>MHHHHHHMIVRRATYEDLSQLAVLFDEYRQFYGASSNLEESHHFLKQRFENKESVFFIHIKDEKITGFVLLYLGFSSVACSTYYILDDVYVTPLFRRQGSAKQLIDTAILFAKQENALRISLETQSNNHESHRLYEKMGFIRDSEFQTFHCFLK[2x]

Here we have uncovered a GNAT-family acetyltransferase conserved in A. baumannii that is responsible for the acetylation of 1,3-DAP in A. baumannii in vivo and in vitro and renamed accordingly as Dpa for diamino-propane acetyltransferase. The crystal structure of Dpa reveals topological and functional differences from other bacterial polyamine acetyltransferases, adopting a β-swapped quaternary arrangement similar to that of eukaryotic polyamine acetyltransferases with a central size exclusion channel that sieves through the cellular polyamine pool. In this study, we have found a downstream regulatory element in this pathway: the polyamine acetyltransferase Dpa that specifically acetylates 1,3-DAP in A. baumannii to control the effective levels of the metabolite. The structure of Dpa revealed a dimeric architecture with a conserved acCoA and an acidic polyamine binding site formed at the dimer interface that shares properties with other polyamine acetyltransferases.

To better understand its structure-function interplay, we determined the structure of Dpa bound to acCoA. Dpa had an overall topology common to GNAT family acetyltransferases. Unlike SpeG acetyltransferases that form higher oligomers, Dpa formed a dimer through a C-terminal β-strand swap. The acidic nature of the channel likely facilitated the access of basic polyamines into the reaction center. The dimensions of the β-swap channel contiguous to the constricted reaction center likely favored the specificity of Dpa for the smaller 1,3-DAP polyamine. The active center of Dpa is very acidic and involves residues Y21, Y25, Y65, Y128, D80, D81, E116. By contrast, in Dpa, Aac(6’)-Iy and PaiA the phosphoadenosine is docked entirely against α-helix α6 due to the divergent sequence of the P-loop, where the first residue in canonic [GxGx(A/G)] motif G is substituted by a large and charged reside. The large R90 sidechain in Dpa pushes the adenosine moiety against the α6 α-helix. In Dpa, like in SSATs, a swapped dimer is formed by the β-strand exchange, while bacterial SpeG-like enzymes adopt large torus-shaped oligomeric structures.>[2x]TPVGLAGFVNKDQIAKDVK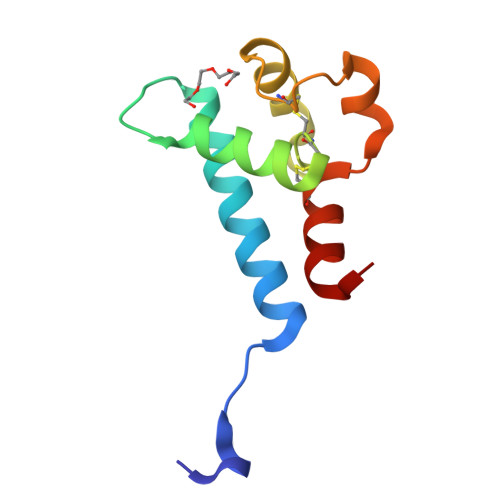QFYDQALQQAVVDDDANNAKAVVKTFHETLNCCGSSTLSALTTSMLKNNLCPSGSSIISNLFKEDCHQKIDELFSGKL>MYDHFNSPSIDILYDYGPFLKKCEMTGGIGSYSAGTPTPRVAIVGAGISGLVAATELLRAGVKDVVLYESRDRIGGRVWSQVFDQTRPRYIAEMGAMRFPPSATGLFHYLKKFGISTSTTFPDPGVVDTELHYRGKRYHWPAGKKPPELFRRVYEGWQSLLSEGYLLEGGSLVAPLDITAMLKSGRLEEAAIAWQGWLNVFRDCSFYNAIVCIFTGRHPPGGDRWARPEDFELFGSLGIGSGGFLPVFQAGFTEILRMVIN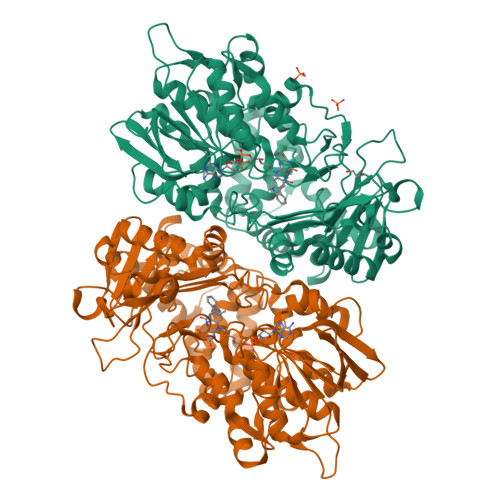GYQSDQRLIPDGISSLAARLADQSFDGKALRDRVCFSRVGRISREAEKIIIQTEAGEQRVFDRVIVTSSNRAMQMIHCLTDSESFLSRDVARAVRETHLTGSSKLFILTRTKFWIKNKLPTTIQSDGLVRGVYCLDYQPDEPEGHGVVLLSYTWEDDAQKMLAMPDKKTRCQVLVDDLAAIHPTFASYLLPVDGDYERYVLHHDWLTDPHSAGAFKLNYPGEDVYSQRLFFQPMTANSPNKDTGLYLAGCSCSFAGGWIEGAVQTALNSACAVLRSTGGQLSKGNPLDCINASYRY[2x]(2R)-2-(5-hydroxy-2-methyl-1H-indol-3-yl)-N-{(1S)-1-[5-(2-methoxyquinolin-3-yl)-1H-imidazol-2-yl]pentyl}propanamide | 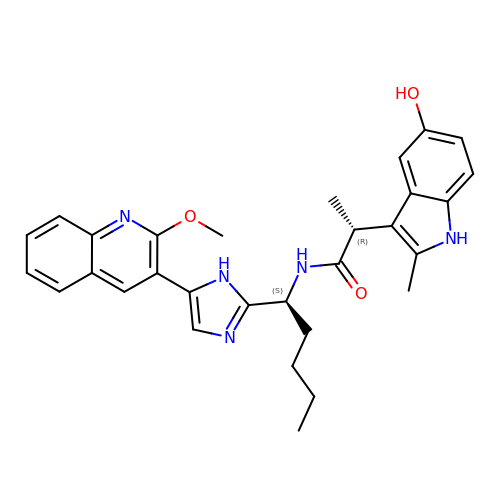C30 H33 N5 O3 | CZYALTGXIQQGCT-NSYGIPOTSA-N> MLFTVTAPKEVYTVDVGSSVSLECDFDRRECTELEGIRASLQKVENDTSLQSER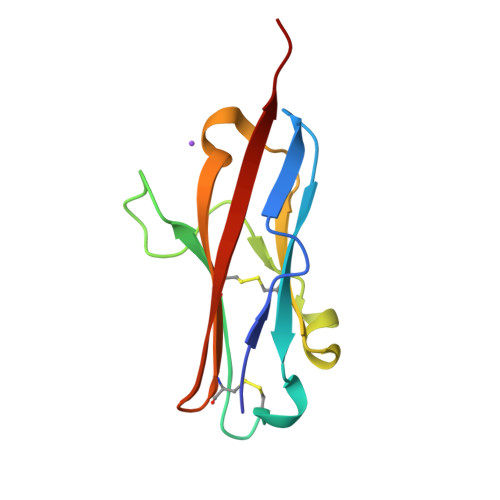ATLLEEQLPLGKALFHIPSVQVRDSGQYRCLVICGAAWDYKYLTVKVKASY>MGSDKIHHHHHHENLYFQGMRYLSKDILEEVITQRPSDSYKSNFGRVVLIGGNRQ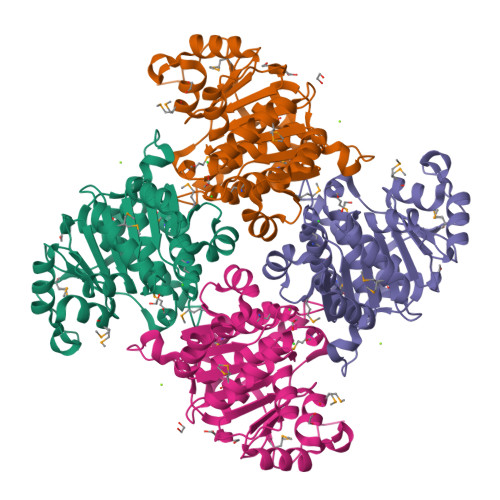YGGAIIMSTEACINSGAGLTTVITDVKNHGPLHARCPEAMVVGFEETVLLTNVVEQADVILIGPGLGLDATAQQILKMVLAQHQKQQWLIIDGSAITLFSQGNFSLTYPEKVVFTPHQMEWQRLSHLPIEQQTLANNQRQQAKLGSTIVLKSHRTTIFHAGEPFQNTGGNPGMATGGTGDTLAGIIAGFLAQFKPTIETIAGAVYLHSLIGDDLAKTDYVVLPTKISQALPTYMKKYAQPHTAPDSELLEQKRSR[2x]>[2x]MRHISPEELIALHD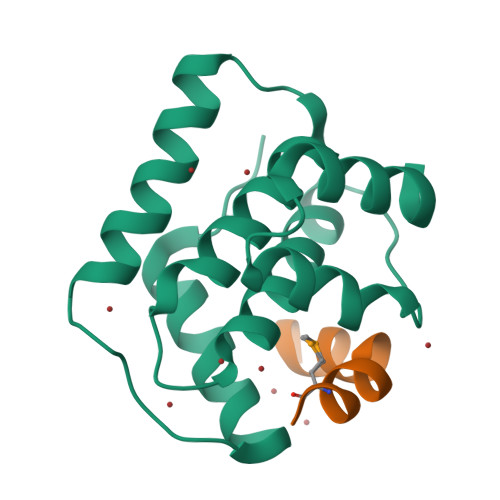ANISRYGGLPGMSDPGRAEAIIGRVQARVAYEEITDLFEVSATYLVATARGYIFNDANKRTALNSALLFLRRNGVQVFDSPELADLTVGAATGEISVSSVADTLRRLYGSADPLEHHHHHH;>ALDAEFASLFDTLDSTNKEMVNR[2x]N-(4-ethoxyphenyl)acetamide | C10 H13 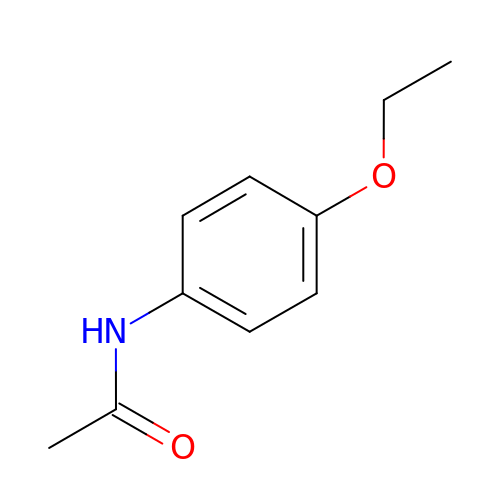N O2 | CPJSUEIXXCENMM-UHFFFAOYSA-N> RNILTNDEGLYGGQSLDVNPYHLIMQEDCNLVLYDHSTAVWSSNTDIPGKKGCKAVLQSDGNFVVYDAEGASLWASHSVRGNGNYVLVLQEDGNVV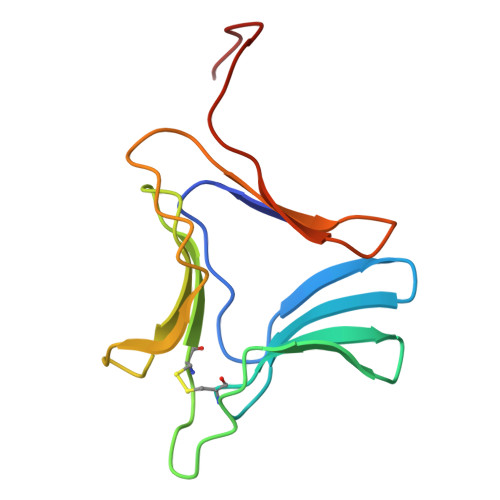IYRSDIWSTNTYR>MKILRFNEGRWGVLEGELVLETDGPGGNPTGRRYDLASVTLLPPATPTKIVCVGRNYREHIREMGHDFGEDLPKEPGLFLKGPNALARPGNPRDPWGTAEPVPYPFFTEELHYEGELAVVVGDRMRHVPPEKALDHVLGYTVAVDITARDVQKKDLQWVRAKSADKFLPLGPWLETDLNPQDTWVRTYVNGTLRQEGHTSQ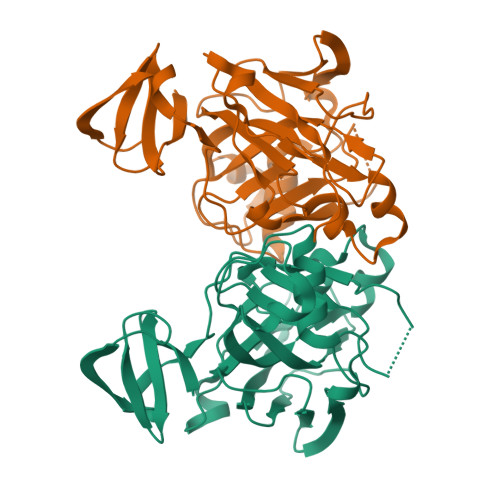MIFSVAEILSYISTFMTLEPLDVVLTGTPEGVGALRPGDRLEVAVEGVGTLFTLIGPKEERPW[4x]>GPGRTNLIVNYLPQNMTQDELRSLFSSIGEVESAKLIRDKVAGHSLGYGFVNYVT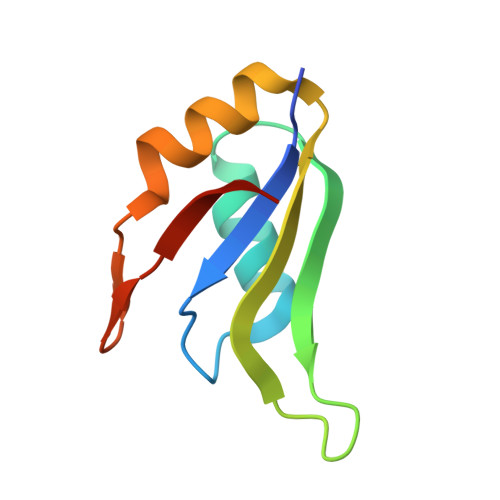AKDAERAINTLNGLRLQSKTIKVSYARPS[4x]>[15x]SFPEVVELNVGGQVYFTRHSTLISIPHSLLWKMF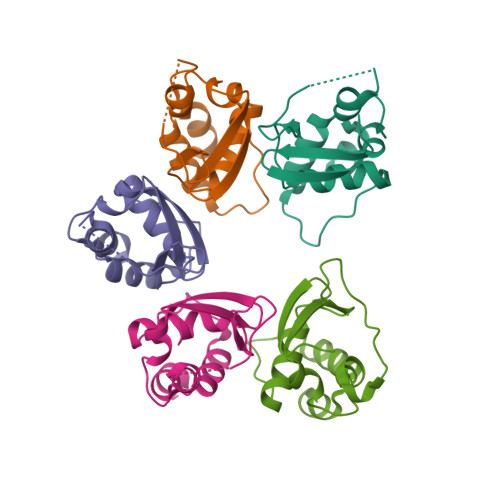SPKRDTANDLAKDSKGRFFIDRDGFLFRYILDYLRDRQVVLPDHFPEKGRLKREAEYFQLPDLVKLLTPDEIKQSPDEF DExD/H-box RNA helicases, from virus and bacteria to eukaryotes, play important roles in processes including ribosome biogenesis, RNA processing and folding, ribonucleoprotein (RNP) remodeling, RNA nuclear export, the regulation of RNA translation and transcription, and nonsense-mediated RNA decay. DExD/H-box proteins often contain accessory regulatory domains and localization modules, but their cores consist of two RecA-like domains joined by a short flexible linker. The N-terminal domain is commonly referred to as conserved domain-1, or DEAD-domain, and the C-terminal domain as conserved domain-2, or helicase domain. Both domains contribute to the binding site for RNA substrates and both contribute to ATP hydrolysis. We used X-ray crystallography to determine the structures of the DEAD-domains of DDX2A, DDX2B, DDX5, DDX10, DDX18, DDX20, DDX47, DDX52, and DDX53, as well as the helicase domains of DDX25 and DDX41.

Also known as eIF4A2, an isoform of DDX2A. Two of the structures show unique P-loop conformations. The DDX2B structure features an α-helix 4 that is longer than in other helicases, and leads into an unusually closed P-loop conformation. As a consequence, the ATP binding site is not visible on the surface of the DDX2B structure. This conformation is most likely induced by a crystal contact in this region.

> MHHHHHHSSGRENLYFQGGVIESNWNEIVDNFDDMNLKESLLRGIYAYGFEKPSAIQQRAIIPCIKGYDVIAQAQSGTGKTATFAISILQQLEIEFKETQALVLAPTRELAQQIQKVILALGDYMGATCHACIGGTNVRNEMQKLQAEAPHIVVGTPGRVFDMLNRRYLSPKWIKMFVLDEADEMLSRGFKDQIYEIFQKLNTSIQVVLLSATMPTDVLEVTKKFMRDPIRILVKKE>MNAHSKEMAPLMGKRTTAPGGNPVVLTEKRPADLTPTKKSAHFFLEIEGFEPNPTVTKTSPPIFSKPMDSNIRQCLSGNCDDMDSPQSPQDDVTETPSNPNSPSANLAKEEQRQKKKRLKKRIFAAVSEGCVEELRELLQDLQDLCRRRRGLDVPDFLMHKLTASDTGKTCLMKALLNINPNTKEIVRILLAFAEENDILDRFINAEYTEEAYEGQTALNIAIERRQGDITAVLIAAGADVNAHAKGVFFNPKYQHEGFYFGETPLALAACTNQPEIVQLLMENEQTDITSQDSRGNNILHALVTVAEDFKTQNDFVKRMYDMILLRSGNWELETMRNNDGLTPLQLAAKMGKAEILKYILSREIKEKPLRSLSRKFTDWAYGPVSSSLYDLTNVDTTTDNSVLEIIVYNTNIDNRHEMLTLEPLHTLLHTKWKKFAKYMFFLSFCFYFFYNITLTLVSYYRPREDEDLPHPLALTHKMSWLQLLGRMFVLIWATCISVKEGIAIFLLRPSDLQSILSDAWFHFVFFVQAVLVILSVFLYLFAYKEYLACLVLAMALGWANMLAYTRGFQSMGMYSVMIQKVILHDVL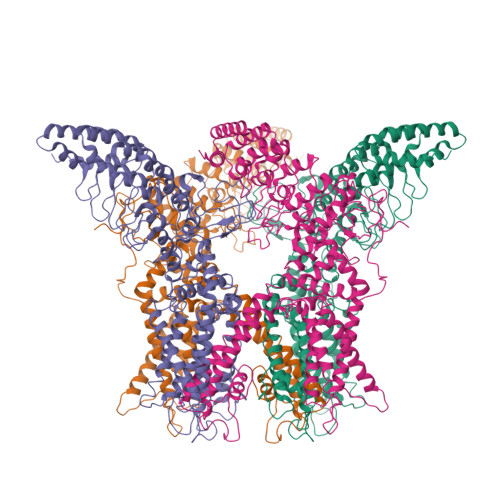KFLFVYILFLLGFGVALASLIEKCSKDKKDCSSYGSFSDAVLELFKLTIGLGDLNIQQNSTYPILFLFLLITYVILTFVLLLNMLIALMGETVENVSKESERIWRLQRARTILEFEKMLPEWLRSRFRMGELCKVADEDFRLCLRINEVKWTEWKTHVSFLNEDPGPIRRTADLNKIQDSSRSNSKTTLYAFDELDEFPETSVLVPRGSAAAWSHPQFEK[4x]>[2x]MKETAAAKFERQHMDSPDLGTLVPRGSMADILSKLLRLGEGRMVKRLKKVADYVGTLSDDVEKLTDAELRAKTDEFKRRLADQKNPETLDDLLPEAFAVAREAAWRVLDQRPFDVQVMGAAALHLGNVAEMKTGEGKTLTCVLPAYLNALAGNGVHI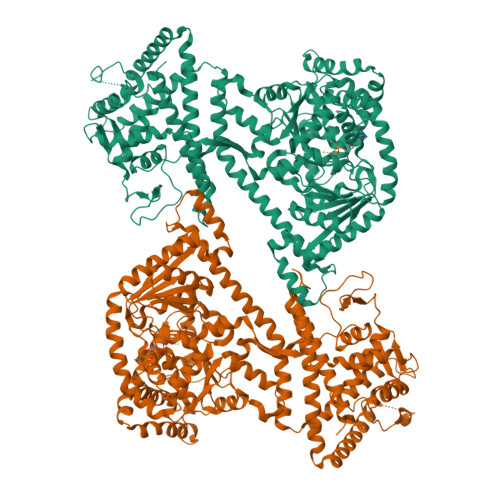VTVNDYLAKRDSEWMGRVHRFLGLQVGVILATMTPDERRVAYNADITYGTNNEFGFDYLRDNMAHSLDDLVQRGHHYAIVDEVDSILIDEARTPLIISGPADGASNWYTEFARLAPLMEKDVHYEVDLRKRTVGVHEKGVEFVEDQLGIDNLYEAANSPLVSYLNNALKAKELFSRDKDYIVRDGEVLIVDEFTGRVLIGRRYNEGMHQAIEAKEHVEIKAENQTLATITLQNYFRLYDKLAGMTGTAQTEAAELHEIYKLGVVSIPTNMPMIREDQSDLIYKTEEAKYIAVVDDVAERYAKGQPVLIGTTSVERSEYLSRQFTKRRIPHNVLNAKYHEQEATIIAVAGRRGGVTVATNMAGRGTDIVLGGNVDFLTDQRLRERGLDPVETPEEYEAAWHSELPIVKEEASKEAKEVIEAGGLYVLGTERHESRRIDNQLRGRSGRQGDPGESRFYLSLGDELMRRFNGAALETLLTRLNLPDDVPIEAKMVTRAIKSAQTQVEQQNFEVRKNVLKYDEVMNQQRKVIYAERRRILEGENLKDQALDMVRDVITAYVDGATGEGYAEDWDLDALWTALKTLYPVGITADSLTRKDHEFERDDLTREELLEALLKDAERAYAAREAELEEIAGEGAMRQLERNVLLNVIDRKWREHLYEMDYLKEGIGLRAMAQRDPLVEYQREGYDMFMAMLDGMKEESVGFLFNVTVEAVPAPPVAPAAEPAELAEFAAAAAAAAQQRSAVDGGARERAPSALRAKGVASESPA> P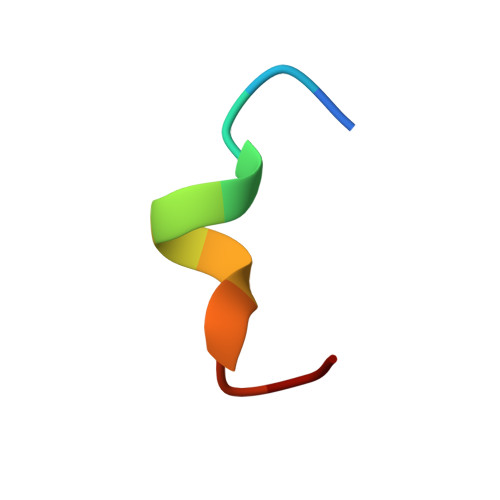INRGDLSRFI>[2x]AYRICLIEGDGIGHEVIPAARRVLEATGLPLEFVEAEAGWETFERRGTSVPEETVEKILSCHATLFGAATSPTRKVPGFFGAIRYLRRRLDLYANVRPAKSRPVPGSRPGVDLVIVRENTEGLYVEQERRYLDVAIADAVISKKASERIGRAALRIAEGRPRKTLHIAHKANVLPLTQGLF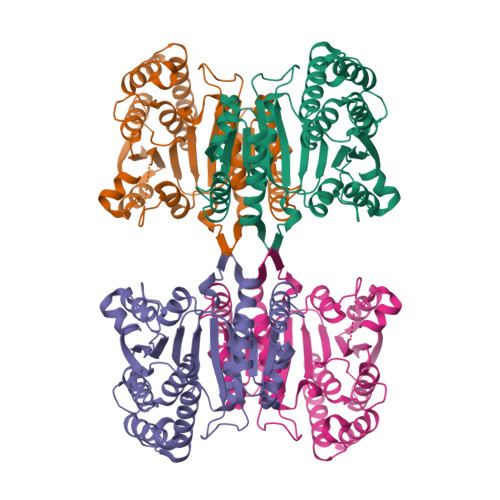LDTVKEVAKDFPLVNVQDIIVDNCAMQLVMRPERFDVIVTTNLLGDILSDLAAGLVGGLGLAPSGNIGDTTAVFEPVHGSAPDIAGKGIANPTAAILSAAMMLDYLGEKEAAKRVEKAVDLVLERGPRTPDLGGDATTEAFTEAVVEALKSL N-[5-(6-ethyl-2,6-diazaspiro[3.3]heptan-2-yl)pyridin-2-yl]-5-fluoro-4-[(4R)-4-methyl-5,6,7,8-tetrahydro-4H-pyrazolo[1,5-a]azepin-3-yl]pyrimidin-2-amine | C25 H31 F N8 | 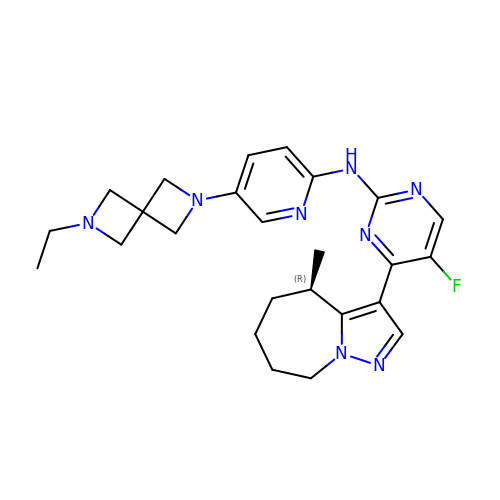KMRYRPPWJDYHAL-QGZVFWFLSA-N> MASMGVPALFRLLSRKFAKVITPVIEAPTEKLPDGTEIEPDLSLPNPNGVECDNLYLDMNGIVHPCSHPEDRPAPETEDEMMVAVFEYTDRILAMVRPRQLLFIAIDGVAPRAKMNQQRSRRFRSSREAALKEEELQAFIEEAKQQGIPIDENATKKKSWDSNCITPGTPFMDTLAKSLRYYIINKLNSDPCWRNVRFILSDASVPGEGEHKIMEFIRSQRVKPEYDPNTHHVVYGLDADLIMLGLATHEPHFRVLREDVFFQQGSTKKTKEERLGIKRLDDVSETNKVPVKKPFIWL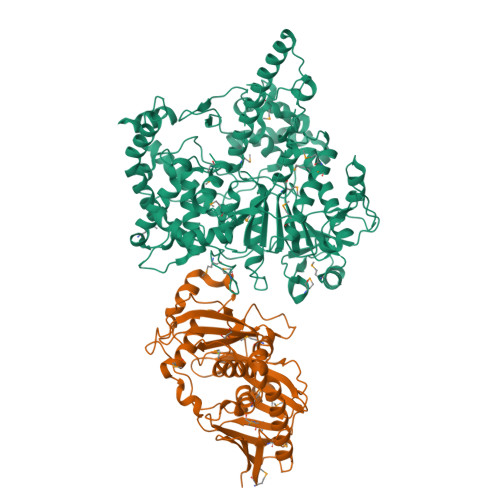NVSILREYLEVELYVPNLPFPFDLERAIDDWVFFIFFVGNDFLPHLPSLDIRDGAVERLTEIWRASLPHMGGYLTLDGSVNLARAEVILSAVGNQEDDIFKRLKQQEDRRNENYRRRQQRESNQESESYVDNVVIQRSVETQSTEVVTSSKSTSVDTKPPKKTQKIDAPAPVDLVNLSEKTSNRSLGATNRELINNRAANRLGLSREAAAVSSVNKLAASALKAQLVSNETLQNVPLEDSIASSSAYEDTDSIESSTPVVHPIDTKVSNVGQKRKAPDSTEENENTDTVRLYEPGYRERYYEQKFHISPDEPEKIREAVKHYVHGLCWVLLYYYQGCPSWTWYYPYHYAPFAADFKDLASIDVKFELNQPFKPYEQLLGVLPAASKNNLPEKLQTLMTDENSEIIDFYPENFTIDLNGKKFEWQGVALLPFIDENRLLNAVSKIYPQLTEEESKRNEDGSTLLFISEHHPMFSELVKQLYSKKRQGKPLKLSGKMAHGLFGKVNTNDSVIPNVSVQCPIDVTSADALQKYGSIDDNQSISLVFEVPKSHFVHKSMLLRGVKMPNRVLTPEDINQVRAERSFSSRRNNGNSAAALEHHHHHH;> MLREFSFYDVPPAHVPPVSEPLEIACYSLSRDRELLLDDSKLSYYYPPPLFSDLNTGFPNRFHPPKSDPDPISIVKDVLMTKGIQMNSSFLTWRGLITKIMCAPLDPRNHWETYLVMDPTSGIIMMEERTRSETSYANQDRMCYWGYKFEAISTLPEIWDACSRDQIEQRDNQDVVPDEQYCSIVKINIGKSKLILAGEVDCIWDKKPCSAKESDVHSDDGTIEEDASNAENPNLHYVELKTSKKYPLENYGMRKKLLKYWAQSFLLGIGRIIIGFRDDNGILIEMKELFTHQIPKMLRPYFKPNDWTPNRLLVVLEHALEWIKQTVKQHPPSTEFTLSYTGGSKLVLRQII> MFERFTDRARRV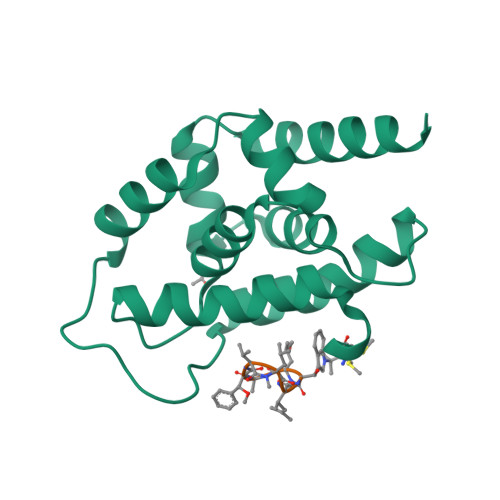VVLAQEEARMLNHNYIGTEHILLGLIHEGEGVAAKSLESLGISLEGVRSQVEEIIGQGQQAPSGHIPYTPRAKKVLELSLREALQLGHNYIGTEHILLGLIREGEGVAAQVLVKLGAELTRVRQQVIQLLSGYLEHHHHHH;> WLAFVLV> MKSVIYHALSQKEANDSDVQPSGAQRAEAFVRAFLKRSTPRMSPQAREDQLQRKAVVLEYFTRHKRKEKKKKAKGLSARQRRELRLFDIKPEQQRYSLFLPLHELWKQYIRDLCSGLKPDTQPQMIQAKLLKADLHGAIISVTKSKCPSYVGITGILLQETKHIFK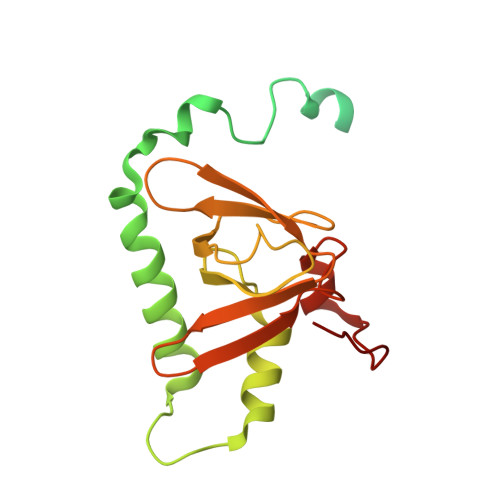IITKEDRLKVIPKLNCVFTVETDGFISYIYGSKFQLRSSERSAKKFKAKGTIDL>FEGDLKWHHHNITYWIQNYSEDLPRAVIDDAFARAFALWSAVTPLTFTRVYSRDADIVIQFGVAEHGDGYPFDGKDGLLAHAFPPGPGIQGDAHFDDDELWSLGKGQGYSLFLVAAHQFGHALGLDHSSVPEALMYPMYRFTEGPPLHKDDVNGIRHL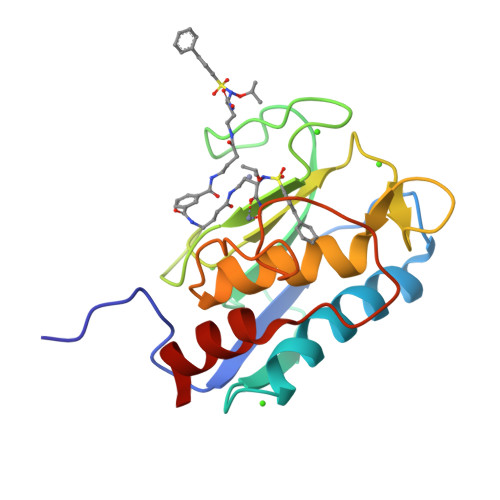YG[2x]>[2x]MNSIQIADETYVAADAARVSAAVADRCSWRRWWPDLRLQVTEDRADKGIRWTVTGALTGT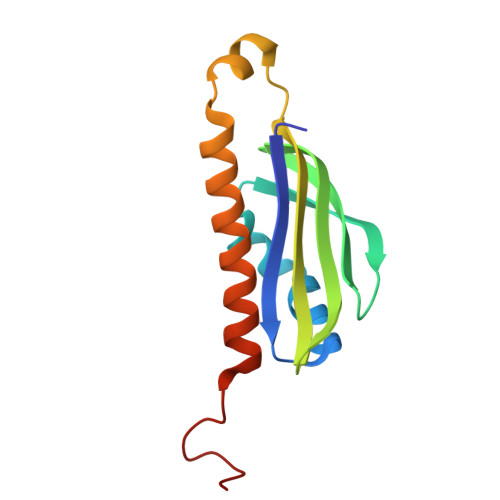MEIWLEPSMDGVLLHYFLHAEPTGVAAWQLARMNLARMTHHRRVAGKKMAFEVKTVLERSRPIGVSPVT> MGSSHHHHHHSQDPMKIDMTEVNNQKTALANSISNLNGQIDTAKNSLTNLTSSSSLTGDVKTAIDAKINNYQV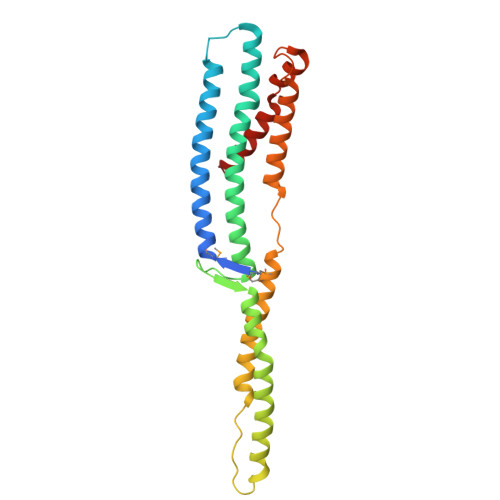PLLTNFTNALTTLSAQYDKTIEQFQSTVSENAADAVIDTDYLQGLLDNYSGIETSISTINTETSTIYSSISDIISLTNPDSSTITTPLAAAKTILTDTKTNMESFNGWTRGTELADLLLSQTQTIETLIGYASSGYTAADAKSFYNNNEFLQGVNKIAEAIANST> SANNPWTGFQIFLSPYYANEVAAAAKQITDPTLSSKAASVANIPTFTWLDSVAKIPDLGTYLASASALGKSTGTKQLVQIVIYDLPDRDCAAKASNGEFSIANNGQANYENYIDQIVAQIQQFPDVRVVAVIEPDSLANLVTNLNVQKCANAKTTYLASVNYALTNLAKVGVYMYMDAGHAGWLGWPANLSPAAQLFTQVWQNAGKSPFIKGLATNVANYNALQAASPDPITQGNPNYDEIHYINALAPLLQQAGWDATFIVDQGRSGVQNIRQQWGDWCNIKGAGFGTRPTTNTGSQFIDSIVWVKPGGESDGTSNSSSPRYDS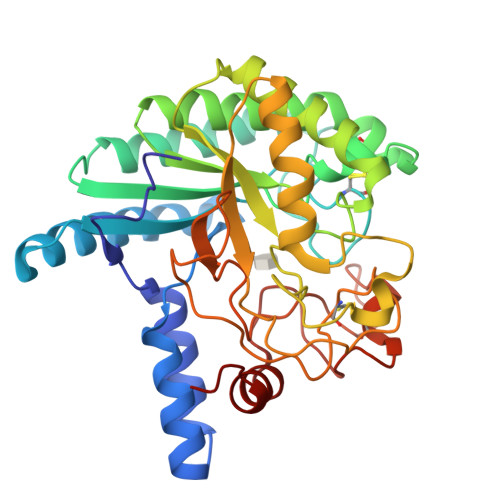TCSLPDAAQPAPEAGTWFQAYFQTLVSAANPPL ZnT8, one of the 10 ZnTs that have been identified so far, is localized in the insulin secretory granules of pancreatic β cells and responsible for the accumulation of high level of zinc inside granules, which is required for the packing of insulin in the hexameric form. ZnT8 functions as a Zn2+/H+ exchanger. The structure of HsZnT8 in the outward-facing state shows a ‘V’-shaped dimeric architecture similar to the crystal structure of EcYiiP, with the two TMDs forming the branches, whereas the two tightly packed CTDs located at the base of the ‘V’ and mediating the majority of the dimerization interactions. Our structural and functional analyses reveal a total of 4 Zn2+ binding sites in each subunit, including one primary site in the TMD (STM), one site at the interface between TMD and CTD (SIF), and two adjacent sites located in an open pocket of CTD covered by a HCH motif from the N-terminal segment of neighboring subunit (SCD1 and SCD2).

Subsequently, we introduced two mutations, D110N and D224N, at the predicted primary Zn2+ binding site within the TMD of HsZnT8 (HsZnT8-DM). As the primary site functions as the transfer center for Zn2+ transport, we reasoned that by abolishing its Zn2+-binding capability, the HsZnT8-DM mutant could potentially stabilize the transporter in a specific state. Indeed, the double mutations appeared to further stabilize the transporter in outward-facing conformation and data collected using HsZnT8-DM sample prepared in the absence of Zn2+ yielded a map of the outward-facing transporter with an improved resolution (~3.8 Å) as compared to HsZnT8-WT, allowing us to build a near complete model containing 302 out of 320 residues for each subunit, with the help of the crystal structure of EcYiiP (Lu et al., 2009; Figure 1—figure supplements 3, 4a). The structure of HsZnT8-DM reveals two adjacent Zn2+ binding sites (designated as SCD1 and SCD2) within each CTD, in a pocket encircled by the U-shaped loop near the C-terminus of the protein right after β3. The EM map shows strong density peaks at both SCD1 and SCD2 that can be assigned to Zn2+ ions. In HsZnT8, Zn2+ ions in both SCD1 and SCD2 are coordinated in a classical tetrahedral geometry with the SCD1 Zn2+ chelated by His52, His54, Cys361, and Cys364, and the SCD2 Zn2+ chelated by Cys53, His301, His318 and Glu352. As the HsZnT8-DM sample was prepared in the absence of Zn2+, the bound Zn2+ ions likely come from the host cells for protein expression and appear to be integral part of the protein with high-affinity binding. From the structure of HsZnT8-WT determined in the presence of Zn2+, we also observed cryo-EM density from a third Zn2+ ion coordinated by His137 and His345 at the interface between CTD and TMD, which is designated as SIF. This Zn2+ density was not present in the HsZnT8-DM structure which was determined in the absence Zn2+, suggesting a lower affinity Zn2+ binding at SIF as compared to the other two CTD sites (SCD1 and SCD2).

>MYHCHSGSKPTEKGANEYAYAKWKLCSASAICFIFMIAEVVGGHIAGSLAVVTDAAHLLINLTSFLLSLFSLWLSSKPPSKRLTFGWHRAEILGALLSILCIWVVTGVLVYLACERLLYPDYQIQATVMIIVSSCAVAANIVLTVVLHQRCLGHNHKEVQANASVRAAFVHALGNLFQSISVLISALIIYFKPEYKIADPICTFIFSILVLASTITILKDFSILLMEGVPKSLNYSGVKELILAVDGVLSVHSLHIWSLTMNQVILSAHVATAASRDSQVVRREIAKALSKSFTMHSLTIQMESPVDQDPDCLFCEDPCD[2x]>GAMDPMICLGLEGTAEKTGVGIVTSDGEVLFNKTIMYKPPKQGINPREAADHHAETFPKLIKEAFEVVDKNEIDLIAFSQGPGLGPSLRVTATVARTLSLTLKKPIIGVNHCIAHIEIGKLTTEAEDPLTLYVSGGNTQVIAYVSKKYRVFGETLDIAVGNCLDQFARYVNLPHPGGPYIEELARKGKKLVDLPYTVKGMDIAFSGLLTAAMRAYDAGERLEDICYSLQEYAFSMLTEITERALAHTNKGEVMLVGGVAANNRLREMLKAMCEGQNVDFYVPPKEFCGDNGAMIAWLGLLMHKNGRWMSLDETKIIPNYRTDMVEVNWIKEIKGKKRKIPVEVNWIKK[3x];>[5x]GAMDPMKAKRVQAKIEIEFPSEDVAKVVYEAVL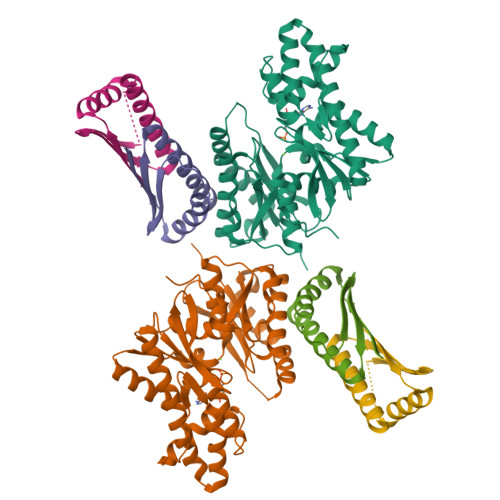YEHLSVPYRRSEIDFKLEGKKIILDIKATDSSALRGTVNSYLRWIKAAIDVIEV>EIDAL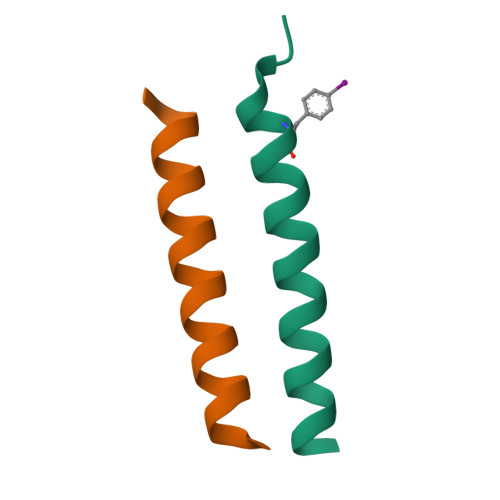EFENDALEQKIAALKQKIASLKQ[2x];>[2x]KIRRLKQKNARLKQEIAALEYEIAALEQ>[2x]MASSASGLRRGHPAGGEENMTETDAFYKREMFDPAEKYKMDHRRRGIALIFNHERFFWHLTLPERRGTCADRDNLTRRFSDLGFEVKCFNDLKAEELLLKIHEVSTVSHTDADCFVCVFLSHGEGNHIYAYDAKIEIQTLTGLFKGD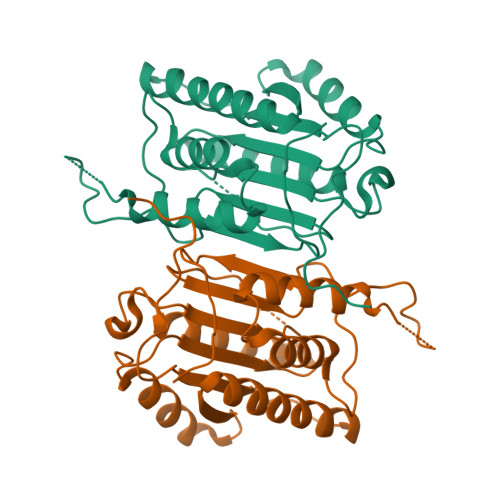KCHSLVGKPKIFIIQACRGNQHDVPVIPLDVVDNQTEKLDTNITEVDAASVYTLPAGADFLMCYSVAEGYYSHRETVNGSWYIQDLCEMLGKYGSSLEFTELLTLVNRKVSQRRVDFCKDPSAIGKKQVPCFASMLTKKLHFFPKSNLEHHHHHH> MYTASGIKAYAQVSVESAVMSASPHQLIEMLFDGANSALVRARLFLEQGDVVAKGEALSKA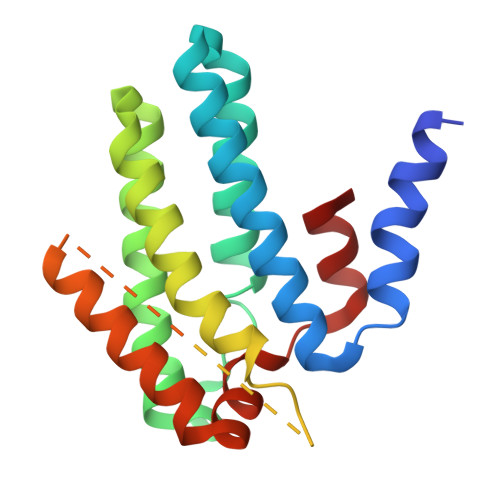INIIDNGLKAGLDQEKGGEIATNLSELYDYMIRRLLQANLRNDAQAIEEVERLLSNIAEAWKQISPKASFQESRGTASGAGGSEGGGSEGGTSGATEDSDYATEVSNMSRAQILQQAGTSVLAQANQVPQNVLSLLR>SLRDQPEQNECQLEHLNALEPDNRIKSEGGLIETWNPSNKQFRCAGVALSRATLQPNSLRRPFYTNAPQEIFIQQGNGYFGMVFPGCVETFEEPRESEQGEGSKFRDSHQKVNRFREGDIIAVPTGVVFWMFNDQDTPVIAVSLIDTSSFQNQLDQMPRRFYLAGNHEQEFLRYQQEGSEEEENEGGNIFSGFKRDFLEDALNVNRRIVNKLQGRNEDEEKGAIVKVKGGLSIITPPEKEPRQKRGSRQEEDEDEDEKRQPHRHSRQDEDEDEKRQPRRHSRGGSKSQRDNGFEETICTARLHQNIGSSSSPDIYNPQAGRIKTVTSFDLPALRFLKLSAEFGSLHKNAMFVPHYNLNANSILYALKGRARLQIVNCKGNSVFDGELEAGRA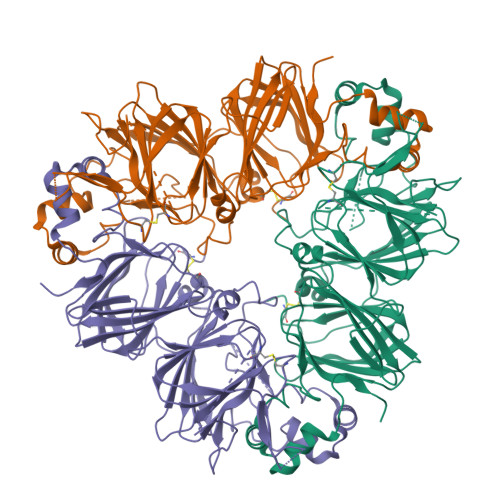LIVPQNFAIAAKSLSDRFSYVAFKTNDRAAIGRLLGASSLINGMPEEVVAAAFNMERNEARQLKFNSPFSFLVPPRSDSDNKAAALE[3x]> SKNEWRKSAIANTLLYLRLKNIYVSADDFVEEQNVYVLPKNLLKKFIEISDVKIQVAAFIYGMSAKDHPKVKEIKTVVLVPQLGHVGSVQISNIPDIGDLPDTEGLELLGWIHTQTEELKFMAASEVATHSKLFADKKRD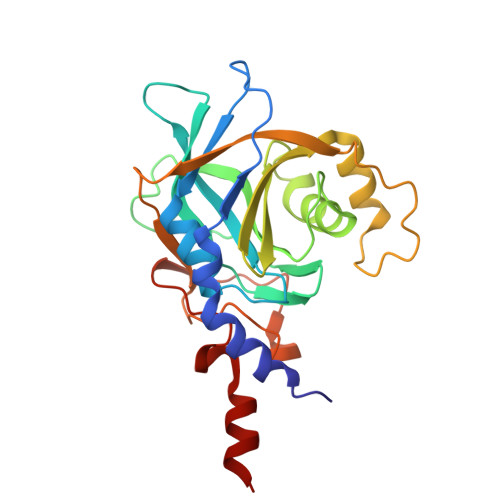CIDISIFSTPGSVSLSAYNLTDEGYQWGEENKDIMNVLSEGFEPTFSTHAQLLLSDRITGNFIIPSGNVWNYTFMGTAFNQEGDYNFKYGIPLEFYNEMHRPVHFLQFSEL>MEEECRVLSIQSHVIRGYVGNRAATFPLQVLGFEIDAVNSVQFSNHTGYAHWKGQVLNSDELQELYEGLRLNNMNKYDYVLTGYTRDKSFLAMVVDIVQELKQQNPRLVYVCDPVLGDKWDGEGSMYVPEDLLPVYKEKVVPLADIITPNQFEAELLSGRKIHSQEEALRVMDMLHSMGPDTVVITSSDLPSPQGSNYLIVLGSQRRRNPAGSVVMERIRMDIRKVDAVFVGTGNLFAAMLLAWTHKHPNNL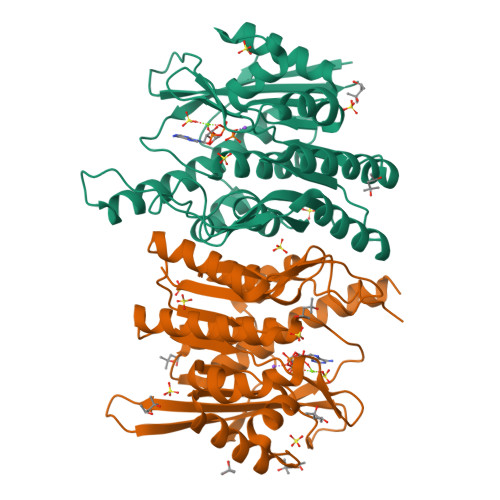KVACEKTVSTLHHVLQRTIQCAKAQAGEGVRPSPMQLELRMVQSKRDIEDPEIVVQATVL[2x]> SPIPVTIREHAGTWYSTLPDSTVPIYGKTPVAPANYMVGEYKDFLEIAQIPTFIGNKVPNAVPYIEASNTAVKTQPLAVYQVTLSCSCLANTFLAALSRNFAQYRGSLVYTFVFTGTAMMKGKFLIAYTPPGAGKPTSRDQAMQATYAIWDLGLNSSYSFTVPFISPTHFRMVGTDQANITNVDGWVTVWQLT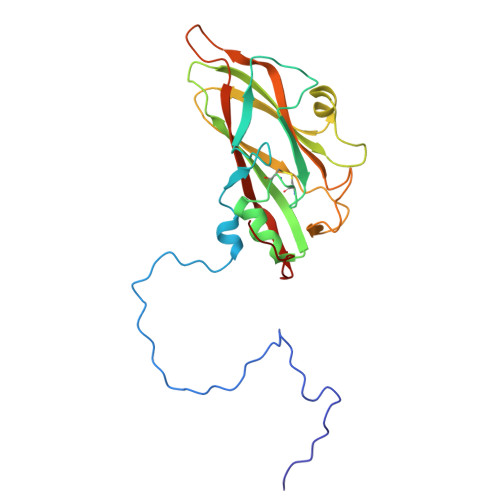PLTYPPGCPTSAKILTMVSAGKDFSLKMPISPAPWSPQ>[2x]GLVPRGSHMAYISLNYHSPTIGMHQNLTVILPEDQSFFNSDTTVKPLKTLMLLHGLSSDETTYMRYTSIERYANEHKLAVIMPNVDHSAYANMAYGHSYYDYILEVYDYVHQIFPLSKKRDDNFIAGHSMGGYGTIKFALT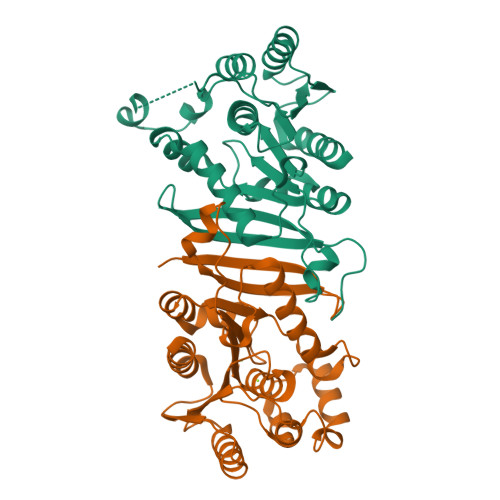QGDKFAKAVPLSAVFEAQNLMDLEWNDFSKEAIIGNLSSVKGTEHDPYYLLDKAVAEDKQIPKLLIMCGKQDFLYQDNLDFIDYLSRINVPYQFEDGPGDHDYAYWDQAIKRAITWMVND> VPPALHLVDPQIQLTITADPKVYPIILRLGSNLSLSMARRNLDSLEARAFQSTPIV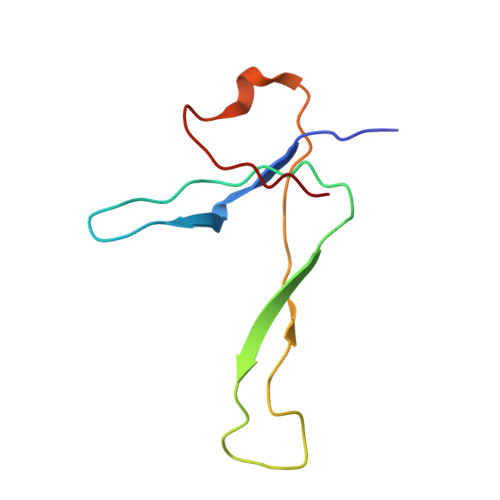VQMTKLATTEELPDEFVVVTAK ethyl 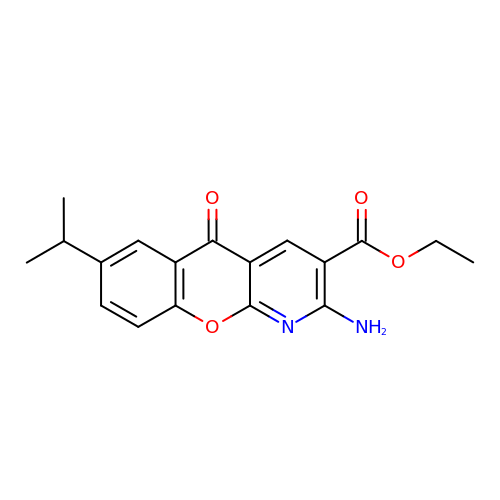2-amino-5-oxo-7-(propan-2-yl)-5H-[1]benzopyrano[2,3-b]pyridine-3-carboxylate | C18 H18 N2 O4 | PFDJAEKKGJFCNL-UHFFFAOYSA-N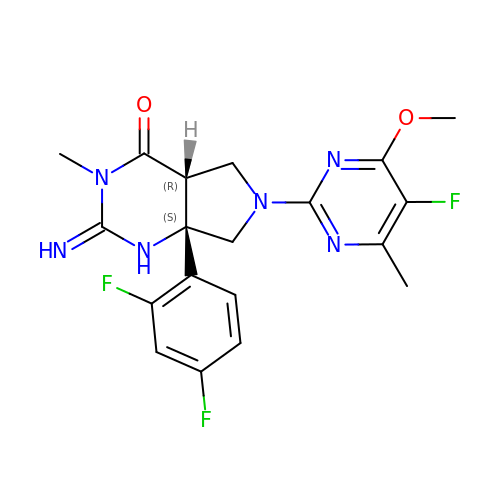(2E,4aR,7aS)-7a-(2,4-difluorophenyl)-6-(5-fluoro-4-methoxy-6-methylpyrimidin-2-yl)-2-imino-3-methyloctahydro-4H-pyrrolo[3,4-d]pyrimidin-4-one | C19 H19 F3 N6 O2 | FNMJFZYRSQTKIH-HXPMCKFVSA-N>MAQIDFRKKINWHRRYRSPQGVKTEHEILRIFESDRGRIINSPAIRRLQQKTQVFPLERNAAVRTRLTHSMEVQQVGRYIAKEILSRLKELKLLEAYGLDELTGPFESIVEMSCLMHDIGNPPFGHFGEAAINDWFRQRLHPEDAESQPLTDDRCSVAALRLRDGEEPLNELRRKIRQDLCHFEGNAQGIRLVHTLMRMNLTWAQVGGILKYTRPAWWRGETPETHHYLMKKPGYYLSEEAYIARLRKELNLALYSRFPLTWIMEAADDISYCVADLEDAVEKRIFTVEQLYHHLHEAWGQHEKGSLFSLVVENAWEKSRSNSLSRSTEDQFFMYLRVNTLNKLVPYAAQRFIDNLPAIFAGTFNHALLEDASECSDLLKLYKNVAVKHVFSHPDVERLELQGYRVISGLLEIYRPLLSLSLSDFTELVEKERVKRFPIESRLFHKLSTRHRLAYVEAVSKLPSDSPEFPLWEYYYRCRLLQDYISGMTDLYAWDEYRRLMAVEQ[6x];>GSFTMGRLYSGNLAAFKAATNKLFQLDLAVIYDDWYDAYTRKDCIRLRI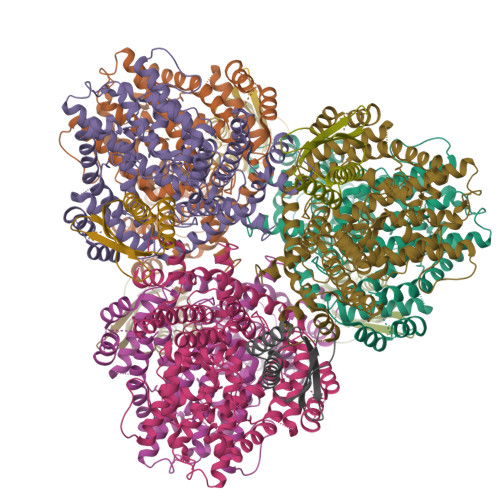EDRSGNLIDTSTFYHHDEDVLFNMCTDWLNHMYDQLKDWK[6x]>MSLQRIVRVSLEHPTSAVCVAGVETLVDIYGSVPEGTEMFEVYGTPGVDIYISPNMERGRERADTRRWRFDATLEIIVVMNSPSNDLNDSHVQISYHSSHEPLPLAYAVLYLTCVDISLDCDLNCEGRQDRNFVDKRQWVWGPSGYGGILLVNCDRDDPSCDVQDNCDQHVHCLQDLEDMSVMVLRTQGPAALFDDHKLVLHTSSYDAKRAQVFHICGPEDVCEAYRHVLGQDKVSYEVPRLHGDEERFFVEGLSFPDAGFTGLISFHVTLLDDSNEDFSASPIFTDTVVFRVAPWIMTPSTLPPLEVYVCRVRNNTCFVDAVAELARKAGCKLTICPQAENRNDRWIQDEMELGYVQAPHKTLPVVFDSPRNGELQDFPYKRILGPDFGYVTREPRDRSVSGLDSFGNLEVSPPVVANGKEYPLGRILIGGNLPGSSGRRVTQVVRDFLHAQKVQPPVELFVDWLAVGHVDEFLSFVPAPDGKGFRMLLASPGACFKLFQEKQKCGHGRALLFQGV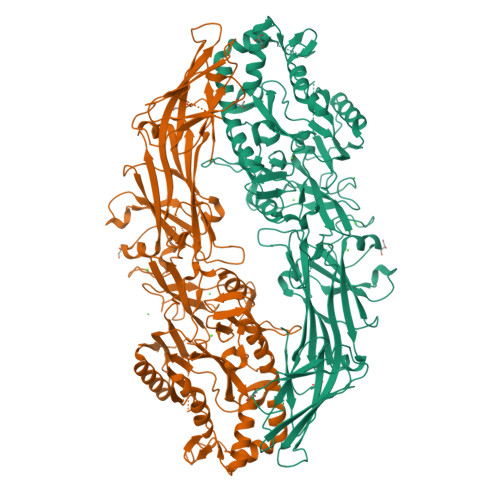VDDEQVKTISINQVLSNKDLINYNKFVQSCIDWNREVLKRELGLAECDIIDIPQLFKTERKKATAFFPDLVNMLVLGKHLGIPKPFGPIINGCCCLEEKVRSLLEPLGLHCTFIDDFTPYHMLHGEVHCGTNVCRKPFSFKWWNMVP[2x]> NALLRYLLD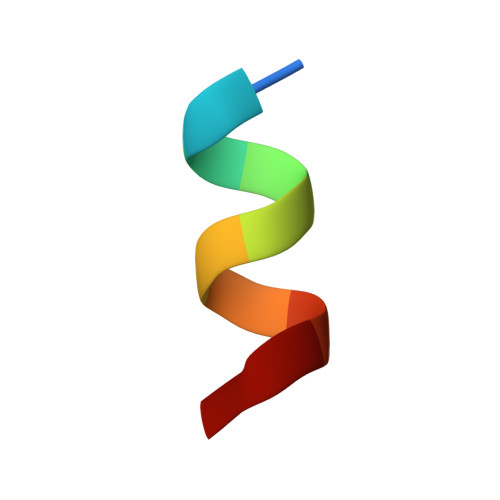K> MQFVNKQFNYKDPVNGVDIAYIKIPNVGQMQPVKAFKIHNKIWVIPERDTFTNPEEGDLNPPPEAKQVPVSYYDSTYLSTDNEKDNYLKGVTKLFERIYSTDLGRMLLTSIVRGIPFWGGSTIDTELKVIDTNCINVIQPDGSYRSEELNLVIIGPSADIIQFECKSFGHEVLNLTRNGYGSTQYIRFSPDFTFGFEESLEVDTNPLLGAGKFATDPAVTLAHELIHAGHRLYGIAINPNRVFKVNTNAYYEMSGLEVSFEELRTF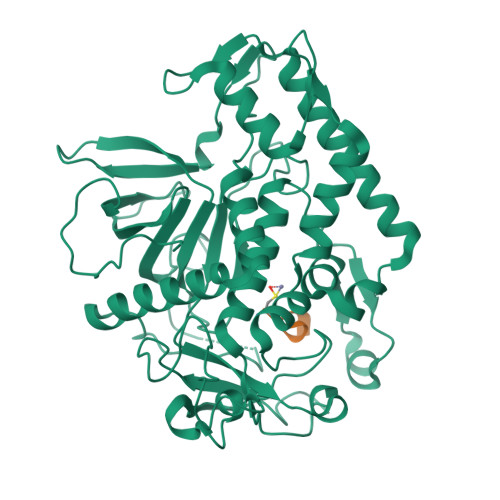GGHDAKFIDSLQENEFRLYYYNKFKDIASTLNKAKSIVGTTASLQYMKNVFKEKYLLSEDTSGKFSVDKLKFDKLYKMLTEIYTEDNFVKFFKVLNRKTYLNFDKAVFKINIVPKVNYTIYDGFNLRNTNLAANFNGQNTEINNMNFTKLKNFTGLFEF;> XCRATKML>[2x]MSIQEIFTKALQDGYLTPAMEAEVGRLCESGVDLDQGEYEALDRLMAALLAGDVVAMPHKKFINVMEEMVLTE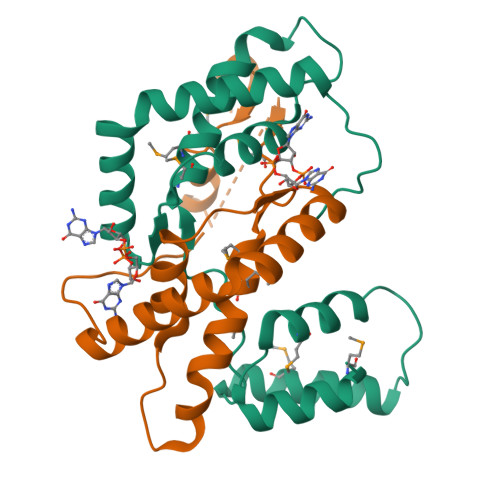VVSQVSKYQKTTEKQPDIADIAAYALNRLPPLYATSEEGAEYQRQRASEELEFLIQQQVKDGLGRYFDRPQIADRKPLEPLVKQDLISQMALLLEALAQDHHHHHH>[5x]SNAEWESITPPVVDAPAVVEFFSFYCPPCYAFSQTMGVDQAIRHVLPQGSRMVKYHVSLLGPLGHELTRAWALAMVMKETDVIE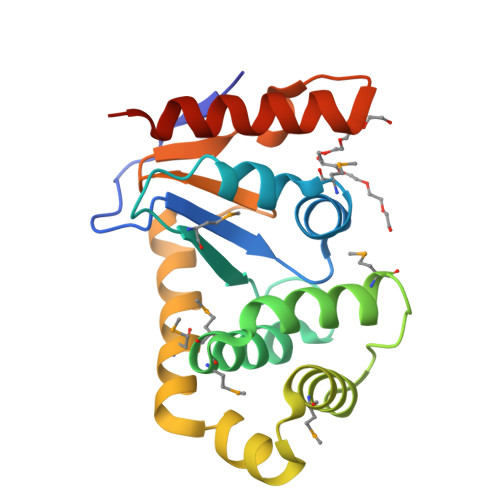KAFFTAGMVEKRLHSPDDVRRVFMSATGISRGEYDRSIKSPAVNDMVALQERLFKEYGVRGTPSVYVRGRYHINNAAFGAFSVENFRSRYAAVVRKLLAGNPDAD S-(D-CARBOXYBUTYL)-L-HOMOCYSTEINE | C9 H17 N 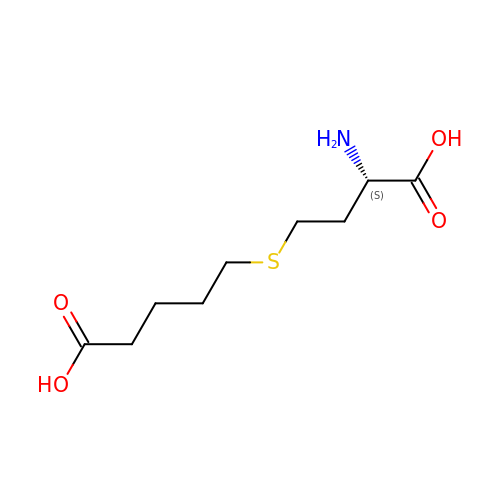O4 S | BMONDXDFXRPNKQ-ZETCQYMHSA-N[5-(4-chlorobenzoyl)-1,4-dimethyl-1H-pyrrol-2-yl]acetic acid | C15 H14 Cl N O3 | 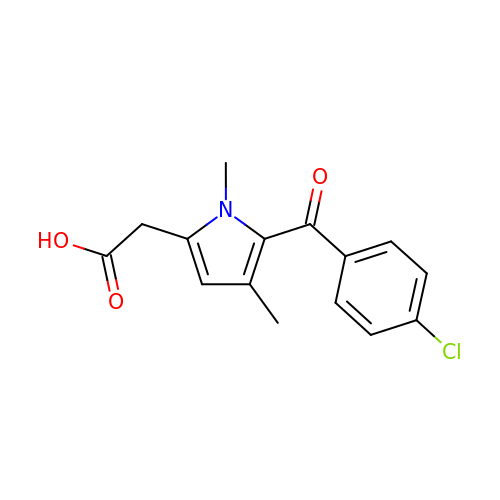ZXVNMYWKKDOREA-UHFFFAOYSA-N1H-INDOLE-3-CARBOXYLIC 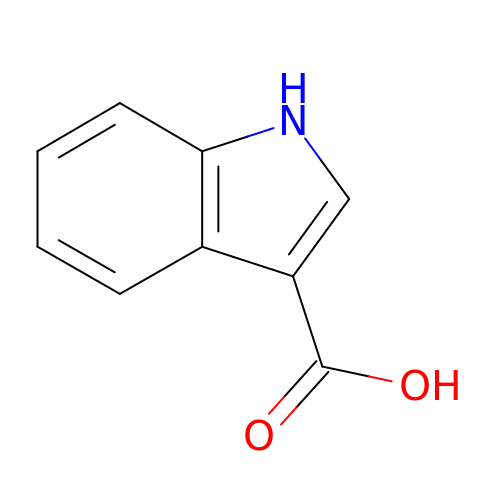ACID | C9 H7 N O2 | KMAKOBLIOCQGJP-UHFFFAOYSA-N methyl beta-D-glucopyranoside | C7 H14 O6 | 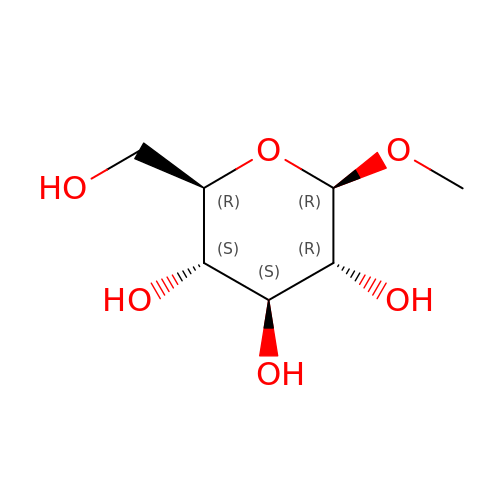HOVAGTYPODGVJG-XUUWZHRGSA-N>MKGPYKHFMQKEIFEQPDSAFNTMRGRIDFENCVVTLGGLKSWLSTIRRCRRIIMIACGTSYHSCLATRSIFEELTEIPVSVELASDFLDRRSPVFRDDTCVFVSQSGETADSILALQYCLERGALTVGIVNSVGSSMSRQTHCGVHINAGPEIGVASTKAYTSQYIALVMFALSLSNDSISRKGRHEEIIKGLQKIPEQIKQVLKLENKIKDLCNSSLNDQKSLLLLGRGYQFATALEGALKIKEISYMHSEGVLAGELKHGILALVDEDLPIIAFATRDSLFPKVMSAIEQVTARDGRPIVICNEGDAIISNDKVHTTLEVPETVDCLQGLLNVIP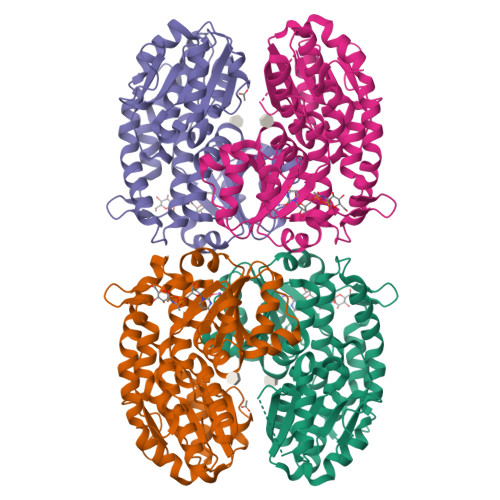LQLISYWLAVNRGIDVDFPRNLAKSVTVE[4x]5-chloranyl-6-fluoranyl-3-(2-propan-2-yloxyphenyl)-1~{H}-indole-2-carboxamide 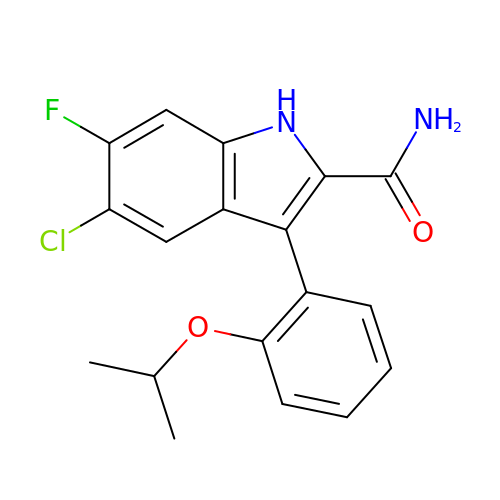| C18 H16 Cl F N2 O2 | CNUHFUPIGPUPON-UHFFFAOYSA-N> RCTRGFRKLGKC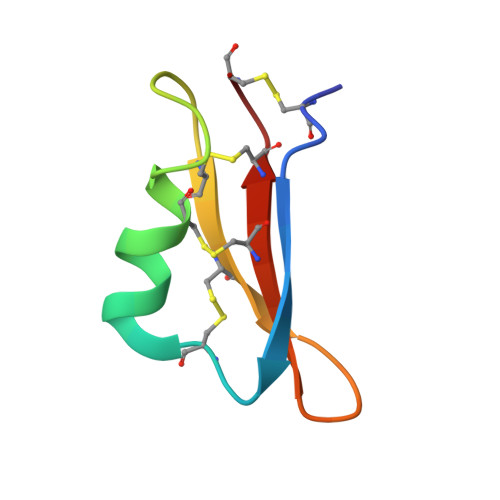TTLEEEKCKTLYPRGQCTCSDSKMNTHSCDCKSC Mammalian reovirus (MRV) is the prototypical member of genus Orthoreovirus of family Reoviridae. Here, we report the 3.3 Å-resolution asymmetric reconstruction of transcribing MRV and in situ atomic models of its capsid proteins, the asymmetrically attached RNA-dependent RNA polymerase (RdRp) λ3, and RdRp-bound nucleoside triphosphatase μ2 with a unique RNA-binding domain. All viruses in the Reoviridae are capable of transcribing RNA inside intact capsids (endogenous transcription) without the need of host factors, an attracting characteristic that allows viral RNA transcription of these viruses to be studied in vitro in cell-free environment. The ISVP transcribes its ten genomic segments, adds a methylated guanosine cap to the 5′ end of each mRNA transcript, and releases the capped mRNA from the turrets at the capsid vertices.

Anchored to each occupied vertex is a TEC, which is a heterodimer composed of one RdRp λ3 and its co-factor μ2 and surrounded by genomic dsRNA. We were able to model 680 of the 736 total amino acid residues of µ2. The atomic model of µ2 has a triangular shape, comprising three domains: an N-terminal, RNA-binding domain20 (RBD, residues 1–264, see details in the TEC–RNA interaction section below), an NTPase domain (residues 265–607) with a bound γ-phosphate group, and a C-terminal domain (CTD, residues 608–736). All three domains of μ2 interact with λ3, with a total contact area of approximately 745 Å2. At the active site of our in situ structure, the priming loop (residues 558–565) extends from the palm domain, blocking the synthesis of double-stranded product, similar to that in the crystal structure of the initiation state. These two features suggest that our in situ structure is at the initiation state. In our structure, the template RNA has already passed through the positively charged entry tunnel to reach the RdRp active site. At the active site near the template RNA is a density that appears to be the putative transcript. Our asymmetric vertex sub-particle reconstruction now further reveals subtle structural differences among the five λ1A/λ1B dimers surrounding each vertex, hereby designated as λ1A1/λ1B1 through λ1A5/λ1B5. Under this convention, λ1A1-2,5/λ1B1-2,5 forms the primary platform to which the TEC binds; by contrast, λ1A3-4/λ1B3-4 make minimal contact, as predicted earlier. Taken together, these structures indicate that the role of N-terminal fragments of λ1A conformers is to anchor the TEC to the capsid and possibly also to regulate transcription. We suggest that CTD guides the template strand of the terminal dsRNA into RdRp to initiate RNA transcription and the NTPase domain provides the required energy for this process, thus playing the role of a helicase, while RBD guides the template RNA out of the RdRp active site.

> MAYIAVPAVVDSRSSEAIGLLESFGVDAGADANDVSYQDHDYVLDQLQYMLDGYEAGDVIDALVHKNWLHHSVYCLLPPKSQLLEYWKSNPSAIPDNVDRRLRKRLMLKKDLRKDDEYNQLARAFKISDVYAPLISSTTSPMTMIQNLNQGEIVYTTTDRVIGARILLYAPRKYYASTLSFTMTKCIIPFGKEVGRVPHSRFNVGTFPSIATPKCFVMSGVDIESIPNEFIKLFYQRVKSVHANILNDISPQIVSDMINRKRLRVHTPSDRRAAQLMHLPYHVKRGASHVDVYKVDVVDMLFEVVDVADGLRNVSRKLTMHTVPVCILEMLGIEIADYCIRQEDGMLTDWFLLLTMLSDGLTDRRTHCQYLINPSSVPPDVILNISITGFINRHTIDVMPDIYDFVKPIGAVLPKGSFKSTIMRVLDSISILGIQIMPRAHVVDSDEVGEQMEPTFEQAVMEIYKGIAGVDSLDDLIKWVLNSDLIPHDDRLGQLFQAFLPLAKDLLAPMARKFYDNSMSEGRLLTFAHADSELLNANYFGHLLRLKIPYITEVNLMIRKNREGGELFQLVLSYLYKMYATSAQPKWFGSLLRLLICPWLHMEKLIGEADPASTSAEIGWHIPREQLMQDGWCGCEDGFIPYVSIRAPRLVIEELMEKNWGQYHAQVIVTDQLVVGEPRRVSAKAVIKGNHLPVKLVSRFACFTLTAKYEMRLSCGHSTGRGAAYSARLAFRSDLA;> MSSMILTQFGPFIESISGITDQSNDVFEDAAKAFSMFTRSDVYKALDEIPFSDDAMLPIPPTIYTKPSHDSYYYIDALNRVRRKTYQGPDDVYVPNCSIVELLEPHETLTSYGRLSEAIENRAKDGDSQARIATTYGRIAESQARQIKAPLEKFVLALLVAEAGGSLYDPVLQKYDEIPDLSHNCPLWCFREICRHISGPLPDRAPYLYLSAGVFWLMSPRMTSAIPPLLSDLVNLAILQQTAGLDPSLVKLGVQICLHAAASSSYAWFILKTKSIFPQNTLHSMYESLEGGYCPNLEWLEPRSDYKFMYMGVMPLSAKYARSAPSNDKKARELGEKYGLSSVVGELRKRTKTYVKHDFASVRYIRDAMACTSGIFLVRTPTETVLQEYTQSPEIKVPIPQKDWTGPIGEIRILKDTTSSIARYLYRTWYLAAARMAAQPRTWDPLFQAIMRSQYVTARGGSGAALRESLYAINVSLPDFKGLPVKAATKIFQAAQLANLPFSHTSVAILADTSMGLRNQVQRRPRSIMPLNVPQQQVSAPHTLTADYINYHMNLSTTSGSAVIEKVIPLGVYASSPPNQSINIDISACDASITWDFFLSVIMAAIHEGVASSSIGKPFMGVPASIVNDESVVGVRAARPISGMQNMIQHLSKLYKRGFSYRVNDSFSPGNDFTHMTTTFPSGSTATSTEHTANNSTMMETFLTVWGPEHTDDPDVLRLMKSLTIQRNYVCQGDDGLMIIDGTTAGKVNSETIQKMLELISKYGEEFGWKYDIAYDGTAEYLKLYFIFGCRIPNLSRHPIVGKERANSSAEEPWPAILDQIMGVFFNGVHDGLQWQRWIRYSWALCCAFSRQRTMIGESVGYLQYPMWSFVYWGLPLVKAFGSDPWIFSWYMPTGDLGMYSWISLIRPLMTRWMVANGYVTDRCSPVFGNADYRRCFNELKLYQGYYMAQLPRNPKKSGRAAPREVREQFTQALSDYLMQNPELKSRVLRGRSEWEKYGAGIIHNPPSLFDVPHKWYQGAQEAAIATREELAEMDETLMRARRHSYSSFSKLLEAYLLVKWRMCEAREPSVDLRLPLCAGIDPLNSDPFLKMVSVGPMLQSTRKYFAQTLFMAKTVSGLDVNAIDSALLRLRTLGADKKALTAQLLMVGLQESEADALAGKIMLQDVNTVQLARVVNLAVPDTWMSLDFDSMFKHHVKLLPKDGRHLNTDIPPRMGWLRAILRFLGAGMVMTATGVAVDIYLEDIHGGGRSLGQRFMTWMRQEGRSA;>YQCHVCSAVLFSPLDLDAHVASHGLHGNMTLTSSDIQRHITEFISSWQNHPIVQVSADVENKKTAQLLHADTPRLVTWDAGLCTSFKIVPIVPAQVPQDVLAYTFFTSSYAIQSPFPEAAVSRIVVHTRWASNVDFDRDSSVIMAPPTENNIHLFKQLLNTETLSVRGANPLMFRANVLHMLLEFVLDNLYLNRHTGFSQDHTPFTEGANLRSLPGPDAEKWYSIMYPTRMGTPNVSKICNFVASCVRNRVGRFDRAQMMNGAMSEWVDVFETSDALTVSIRGRWMARLARMNINPTEIEWALTECAQGYVTVTSPYAPSVNRLMPYRISNAERQISQIIRIMNIGNNATVIQPVLQDISVLLQRISPLQIDPTIISNTMSTVSESTTQTLSPASSILGKLRPSNSDFSSFRVALAGWLYNGVVTTVIDDSSYPKDGGSVTSLENLWDFFILALALPLTTDPCAPVKAFMTLANMMVGFETIPMDNQIYTQSRRASAFSTPHTWPRCFMNIQLISPIDAPILRQWAEIIHRYWPNPSQIRYGAPNVFGSANLFTPPEVLLLPIDHQPANVTTPTLDFTNELTNWRARVCELMKNLVDNQRYQPGWTQSLVSSMRGTLDKLKLIKSMTPMYLQQLAPVELAVIAPMLPFPPFQVPYVRLDRDRVPTMVGVTRQSRDTITQPALSLSTTNTTVGVPLALDARAITVALLSGKYPPDLVTNVWYADAIYPMYADTEVFSNLQRDMITCEAVQTLVTLVAQISETQYPVDRYLDWIPSLRASAATAATFAEWVNTSMKTAFDLSDMLLEPLLSGDPRMTQLAIQYQQYNGRTFNIIPEMPGSVIADCVQLTAEVFNHEYNLFGIARGDIIIGRVQSTHLWSPLAPPPDLVFDRDTPGVHIFGRDCRISFGMNGAAPMIRDETGLMVPFEGNWIFPLALWQMNTRYFNQQFDAWIKTGELRIRIEMGAYPYMLHYYDPRQYANAWNLTSAWLEEITPTSIPSVPFMVPISSDHDISSAPAVQYIISTEYNDRSLFCTNSSSPQTIAGPDKHIPVERYNILTNPDAPPTQIQLPEVVDLYNVVTRYAYETPPITAVVMGVP[10x];>[5x]MKRIPRKTKGKSSGKGNDSTERADDGSSQLRDKQNNKAGPATTEPGTSNREQYKARPGIASVQRATESAEMPMKNNDEGTPDKKGNTKGDLVNEHSEAKDEADEATKKQAKDTDKSKAQVTYSDTGINNANELSRSGNVDNEGGSNQKPMSTRIAEATSAIVSKHPARVGLPPTASSGHG> GPLGSIKELAVDEELAAADGLIPRQKSKLCKHGDRGMCEYCSPLPPWDKEYHEKNKIKHISFHSYLKKLNENANKKENGSSYISPLSEPDFRINKRCHNGHEPWPRGICSKCQPSAITLQQQEFRMVDHVEFQKSEIINEFIQAWRYTGMQRFGYMYGSYSKYDNTPLGIKAVVEAIYEPPQHDEQDGLTMDVEQVKNEMLQIDRQAQEMGLSRIGLIFTDLSDAGAGDGSVFCKRHKDSFFLSSLEVIMAARHQTRHPNVSKYSEQGFFSSKFVTCVISGNLEGEIDISSYQVSTEAEALVTADMISGSTFPSMAYINDTTDERYVPEIFYMKSNEYGITVKENAKPAFPVDYLLVTLTHGFPNTDTETNSKFVSSTGFPWSNRQAMGQSQDYQELKKYLFNVASSGDFNLLHEKISNFHLLLYINSLQILSPDEWKLLIESAVKNEWEESLLKLVSSAGWQTLVMILQESG

Polyubiquitylated proteins in isolation can be direct targets of the proteasome, whereas those embedded into membranes or assembled into multisubunit complexes need to be extracted or segregated by the conserved AAA-family ATPase Cdc48 (yeast) or p97/VCP (metazoan) with the aid of its cofactor complex, Ufd1–Npl4 (UN), prior to the proteasomal degradation. The UN heterodimer is one of the best-characterized cofactors. Here, we present the crystal structures of yeast Npl4 (zf-Npl4-MPN-CTD) in complex with Lys48-linked diubiquitin (K48-Ub2) and with Ufd1 at 2.55 and 1.58 Å resolutions, respectively. The crystal structures reveal that the distal and proximal Ub (Ubdist and Ubprox, respectively) moieties of K48-Ub2 interact with the C-terminal helix and N-terminal loop (N loop) of Npl4 CTD, respectively, and that Ufd1 binds to the groove of Npl4 corresponding to the catalytic groove of JAMM.

The region containing residues 113–580 of Saccharomyces cerevisiae Npl4 (yNpl4113–580, with the prefix “y” indicating Saccharomyces cerevisiae proteins) specifically recognizes K48 chains in vitro. The triple E123A K124A E125A mutation was introduced to reduce excess surface conformational entropy. The yNpl4113–580 (E123A K124A E125A) protein yielded high-quality crystals, and its structure was determined at 1.72 Å resolution by the single-wavelength anomalous diffraction (SAD) method using the zinc edge. The yNpl4113–580 structure consists of three subdomains, zf-Npl4, MPN, and CTD, similarly to the previously reported structures of Npl4. The yNpl4 MPN subdomain consists of the MPN core and two insertions, Ins-1 (residues 287–317) and Ins-2 (residues 403–462), similarly to other MPN DUBs.4-[[(1~{S})-1-[2,5-bis(fluoranyl)phenyl]ethyl]amino]-5-chloranyl-2-fluoranyl-~{N}-(1,3-thiazol-4-yl)benzenesulfonamide 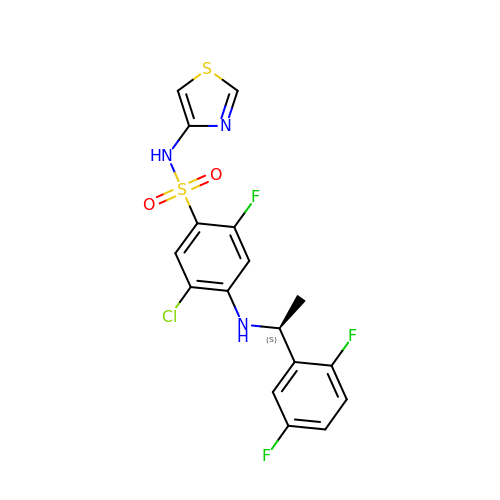| C17 H13 Cl F3 N3 O2 S2 | KLWKJFRXLGLTIH-VIFPVBQESA-N>[2x]SNAMLRRLFKKKYVCVRQYDLTDCGAACLSSIAQYYGLKMSLAKIREMTGTDTQGTNAYGLIHAAKQLGFSAKGVKASKEDLLKDFRLPAIANVIVDNRLAHFVVIYSIKNRIITVADPGKGIVRYSMDDFCSIWTGGLVLLEPGEAFQKGDYTQNMMVKFAGFLKPLKKTVLCIFLASLLYTALGIAGSFYIKFLFDDLIKFEKLNDLHIISAGFAVIFLLQIFLNYYRSILVTKLGMSIDKSIMMEYYSHVLKLPMNFFNSRKVGEIISRFMDASKIRQAISGATLTIMIDTIMAVIGGILLYIQNSSLFFISFIIILLYGIIVTVFNKPIQNANRQIMEDNAKLTSALVESVKGIETIKSFGAEEQTEKSTRDKIETVMKSSFKEGMLYINLSSLTGIVAGLGGIVILWAGAYNVIKGNMSGGQLLAFNALLAYFLTPVKNLIDLQPLIQTAVVASNRLGEILELATEKELREDSDDFVISLKGDIEFR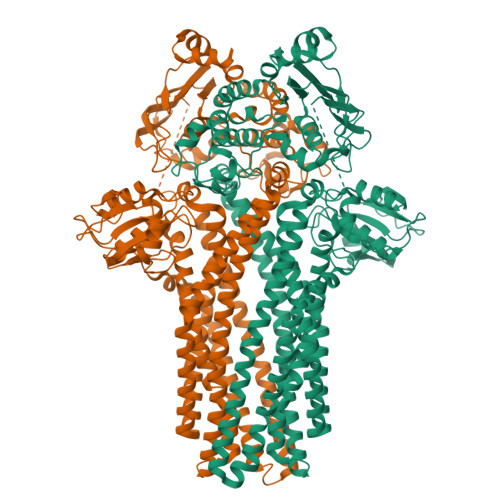NVDFRYGLRKPVLKNINLTIPKGKTVAIVGESGSGKTTLAKLLMNFYSPEKGDILINGHSIKNISLELIRKKIAFVSQDVFIFSGTVKENLCLGNENVDMDEIIKAAKMANAHDFIEKLPLKYDTFLNESGANLSEGQKQRLAIARALLKKPDILILDEATSNLDSITENHIKDAIYGLEDDVTVIIIAHRLSTIVNCDKIYLLKDGEIVESGSHTELIALKGCYFKMWKQTENTLAS>MVMKQTKQTNILAGAAVIKVLEAWGVDHLYGIPGGSINSIMDALSAERDRIHYIQVRHEEVGAMAAAADAKLTGKIGVCFGSAGPGGTHLMNGLYDAREDHVPVLALIGQFGTTGMNMDTFQEMNENPIYADVADYNVTAVNA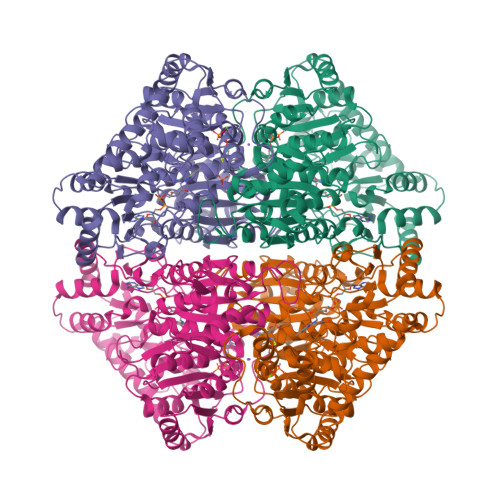ATLPHVIDEAIRRAYAHQGVAVVQIPVDLPWQQIPAEDWYASANSYQTPLLPEPDVQAVTRLTQTLLAAERPLIYYGIGARKAGKELEQLSKTLKIPLMSTYPAKGIVADRYPAYLGSANRVAQKPANEALAQADVVLFVGNNYPFAEVSKAFKNTRYFLQIDIDPAKLGKRHKTDIAVLADAQKTLAAILAQVSERESTPWWQANLANVKNWRAYLASLEDKQEGPLQAYQVLRAVNKIAEPDAIYSIDVGDINLNANRHLKLTPSNRHITSNLFATMGVGIPGAIAAKLNYPERQVFNLAGDGGASMTMQDLATQVQYHLPVINVVFTNCQYGWIKDEQEDTNQNDFIGVEFNDIDFSKIADGVHMQAFRVNKIEQLPDVFEQAKAIAQHEPVLIDAVITGDRPLPAEKLRLDSAMSSAADIEAFKQRYEAQDLQPLSTYLKQFGLDDLQHQIGQGGF[2x]> K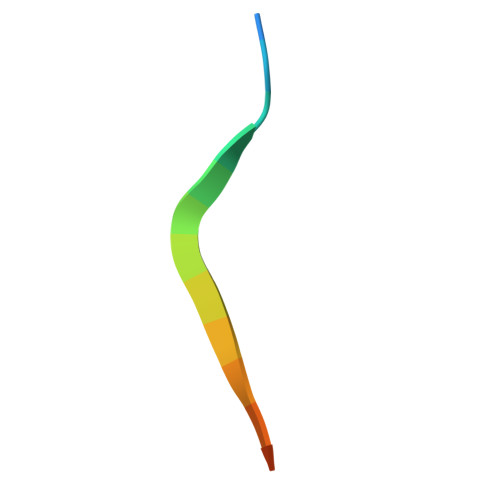GSVVIVGRIILSGRK>[2x]RRIRRPFSVAEVEALVEAVEHLGTGRWRDVKMRAFDNADHRTYVDLKDKWKT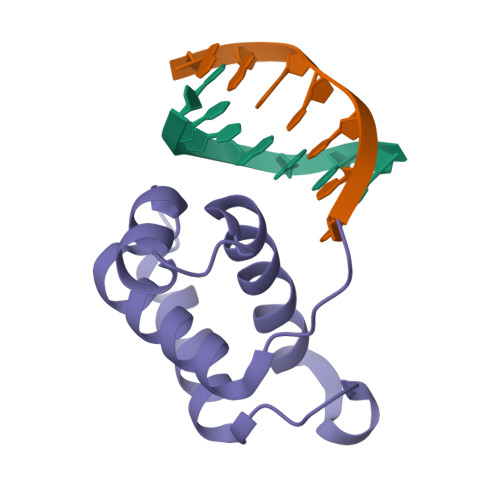LVHTASIAPQQRRGEPVPQDLLDRVLAAHAYWSQ> MGSSHHHHHHSSGLVPRGSHIMQTTIRSAGAMPANRRTSLAQCLALSLALLANAAHAQEVRKAADGVTVVPSAKGAAPVRLQVVDAGIIRVSADPDGDFARSPSLMRVPVQGDTAFQVAEQGDSVQLKTGKVTASISTVDGHVSFADANGKPVLSEVAGGRSFAPLNVEGKQYLSVRQRFQSPDDEALYGFGQHQQGWMNQKGRNVELQQNNIDMAVPYLVSSRNYGLLWDNNSITRLGDPRGLQPLPKTLTLYDAKGKAGALTARYAINGKHILERRESEVNYQYLSDLTKYPKKAITKDKNSRMQVTWEGEIEVLTGGEHTFSLYSSEYAKLYVDGKLVVDRWRQNWNPWNHEFKLDLEPGQRHTVKVEWDLIDPSYIALLHRDPLPAAEAKDLSLWSEAGQMIDYYFVSADSYDQAVAGYRALTGKSTMLPKWAYGFWQSRERYKSQDELVGAVAEYRKRKLSLDNIVLDWSYWPENAWGSHDFDPQHFPDPDGMVKAVHDMHAQIMISIWPKFYPTTANYKELDAAGFMFKRNVEVGELDWIGKGYKNSFYDPYSEKAQAIYWRQINEKLNSKGFDAWWMDADEPDVHSNLDIAERKARTTPNALGSSTEYFNSYPLPHTHGVYVGDRAADDKRVFILSRKGYAGTQRNAVAVWSGDIVSRWDDMRDQISGGVNMALSGLPNWTFDIGGFAVEKRYEDQDPAHLPEWRELNTRWFQFGAFVPIFRSHGQFPYREIWNIAPEGTPFYESMAYYNRLRSALLPYIYSLAGDTYQRDGVIMRGMMMDFPNDPKVRDINDQYLFGPAFLVAPVTRFGATSRQVYLPAGSSWLEFATGKRYEGGQSIEAAAPIERMPLFVRAGSIVPTGPVQEYVDQV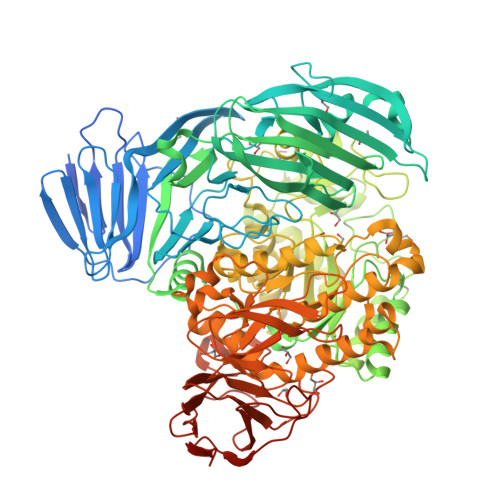ADAPLTVVVYTGADGQFSLYEDDGKGYGYEKGEFSRIPLVWNQAKGELSIGKREGSWTGMQAKRTINVRFVDGPRDDAGALAPKTDASIQYDGKPVSVLQRKIASGKARRR> MLKHIISAYNFSRDELEDIFALTD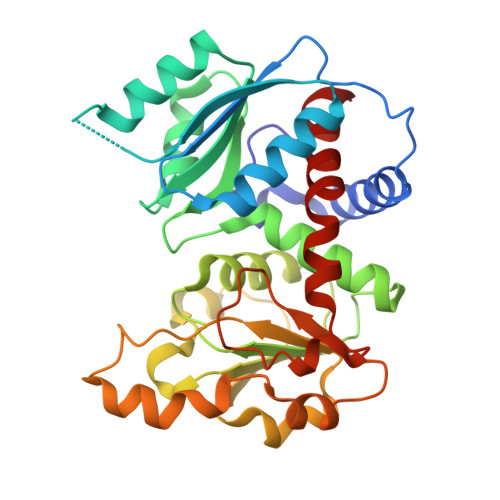KYSKNLNDTRKILSGKTISIAFFEPSTRTYLSFQKAIINLGGDVIGFSGEESTSVAKGENLADTIRMLNNYSDGIVMRHKYDGASRFASEISDIPVINAGDGKHEHPTQAVIDIYTINKHFNTIDGLVFALLGDLKYARTVNSLLRILTRFRPKLVYLISPQLLRARKEILDELNYPVKEVENPFEVINEVDVLYVTRIQKERFVDEMEYEKIKGSYIVSLDLANKMKKDSIILHPLPRVNEIDRKVDKTTKAKYFEQASYGVPVRMSILTKIYGE>GSHMDVVRTKIPMMNIALSGEITGGMQSGLLILAGPSKSFKSNFGLTMVSSYMRQYPDAVCLFYDSEFGITPAYLRSMGVDPERVIHTPVQ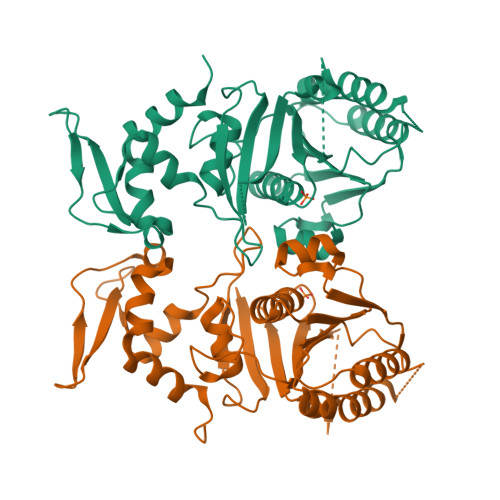SLEQLRIDMVNQLDAIERGEKVVVFIDSLGNLASKKETEDALNEKVVSDMTRAKTMKSLFRIVTPYFSTKNIPCIAINHTYETQEMFSKTVMGGGTGPMYSADTVFIIGKRQIKDGSDLQGYQFVLNVEKSRTVKEKSKFFIDVKFDGGIDPYSGLLDMALELGFVVKPKNGWYAREFLDEETGEMIREEKSWRAKDTNCTTFWGPLFKHQPFRDAIKRAYQLGAIDSNEIVEAEVDELINS[2x]(2R)-N-[(2S,3R)-1-(1,3-benzodioxol-5-yl)-4-{[(4'S)-6'-(2,2-dimethylpropyl)-3',4'-dihydrospiro[cyclobutane-1,2'-pyrano[2,3-b]pyridin]-4'-yl]amino}-3-hydroxybutan-2-yl]-2-methoxypropanamide | C31 H43 N3 O6 | 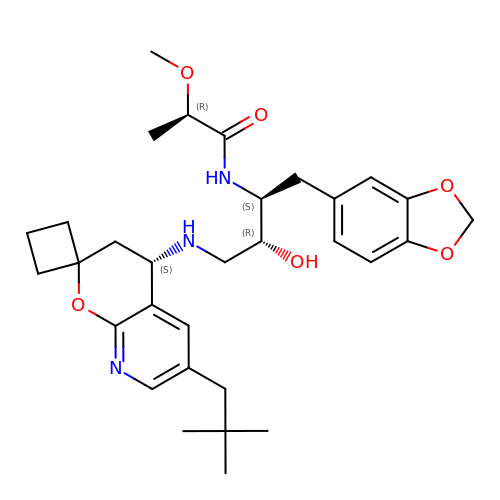OMMVFRZSBCRMQD-LJYZBVLISA-N> VRIRRAGLEDLPGVARVLVDTWRATYRGVVPEAFLEGLSYEGQAERWAQRLKTPTWPGRLFVAESESGEVVGFAAFGPDRASGFPGYTAELWAIYVLPTWQRKGLGRALFHEGARLLQAEGYGRM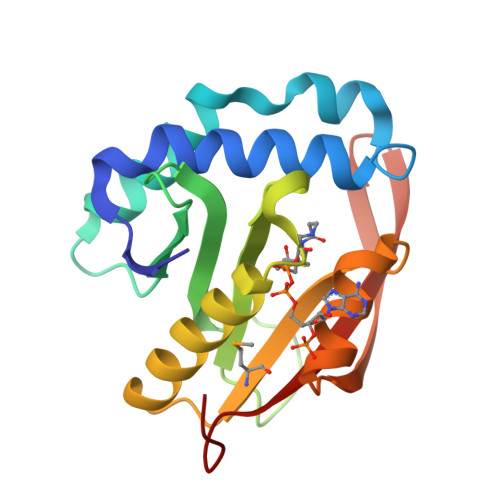LVWVLKENPKGRGFYEHLGGVLLGEREIELGGAKLWEVAYGFDLGGHKW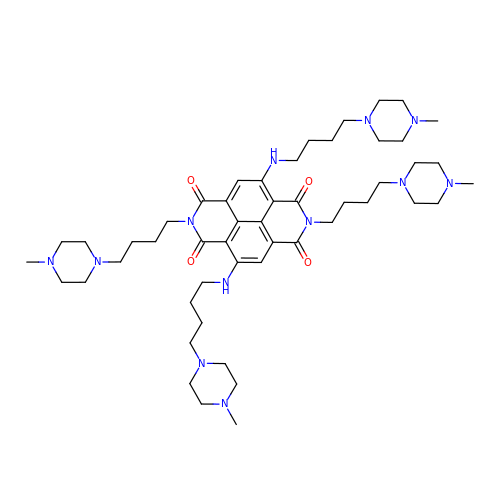2,7-bis[4-(4-methylpiperazin-1-yl)butyl]-4,9-bis{[4-(4-methylpiperazin-1-yl)butyl]amino}benzo[lmn][3,8]phenanthroline-1,3,6,8(2H,7H)-tetrone | C50 H80 N12 O4 | ZQKCDGPBUJAXIX-UHFFFAOYSA-N>MSLAESAFSERIVQNLLDTDFYKLTMMQAVLHNYPNAEVEWEFRCRNQEDLRLYLPAIREQLEYLAGLAISDEQLAFLERIPFLAPDFIRFLGLFRFNPRYVQTGIENDEFFLRLKGPWLHVILFEVPLLAMISEVRNRARYPAATVEQARERLQEKFDWLRREASAEELAGFKMADFGTRRRFSYRVHEAVVSGLKEDFPGCFVGTSNVHLARKLDLKPLGTMAHEWLMAHQQLGPRLIDSQSAALDCWVREYRGLLGIALTDCITTDAFLRDFDLYFAKLFDGLRHDSGDPLLWAEKTIAHYLKLGIDPLTKTLVFSDGLDLPRALKIYRALQGRINVSFGIGTHFTCDLPGVEPMNIVVKM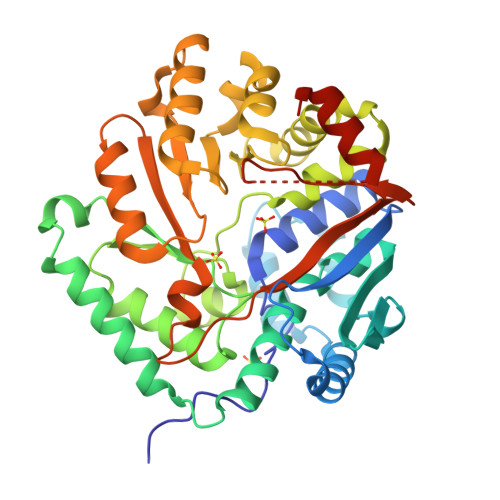SACNGHPVAKISDTPGKAQCRDPDFIHYLKHVFQVAEGHHHHHH[4x]> HFQLQWPGARGAFVANDEVYFCGAHNNVTTNRTDFPLDGSGFVSIKSGHAPYTVGAIISLETDADAWEDFKNSSGGDQIAIAYRQVDNSGTYCVPFNPSSLNIAGIQDGANATIQVVYTGGDGNLYQCADVTFR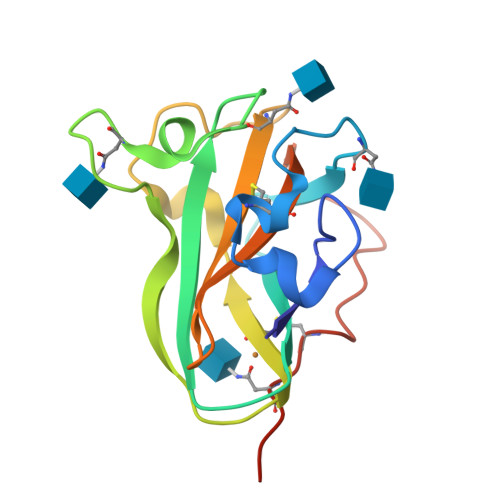TTVANLNSSVCTNSTHHHHHH>[2x]VASPAIVEAKPVKTIKDKVRAMREL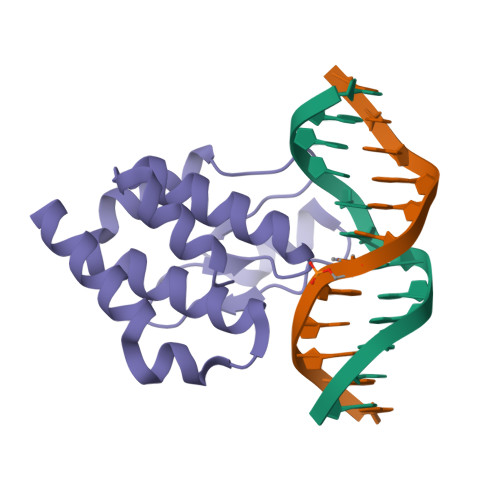LLSDEYAEQKRAVNRFMLLLSTLYSLDAQAFAEATESLHGRTRVYFAADEQTLLKNGNQTKPKHVPGTPYWVITNTNTGRKCSMIEHIMQSMQFPAELIEKVCGTI>[2x]MSLTEYVHGYSEREALRLSEQAETLEKLLHHDTVYPPGAKVLEAGCGIGAQTVILAKNNPDAEITSIDI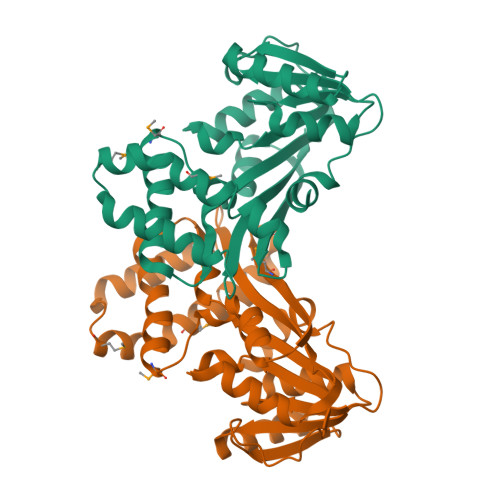SPESLEKARENTEKNGIKNVKFLQANIFSLPFEDSSFDHIFVCFVLEHLQSPEEALKSLKKVLKPGGTITVIEGDHGSCYFHPEGKKAIEAWNCLIRVQAYMKGNSLVGRQIYPLLQESGFEKIRVEPRMVYIDSSKPELVDGFILKTIIPMVEGVKEQSLKMQIIKEEEWEKGIEELHKTAEHGGTFCYTFFKGWGTKEGHHHHHH> MNDQEKIDKFTHSYINDDFGLTIDQLVPKVKGYGRFNVWLGGNESKIRQVLKAVKEIGVSPTLFAVYEKNEGFSSGLGWLNHTSARGDYLTDAKFIARKLVSQSKQAGQPSWYDAGNIV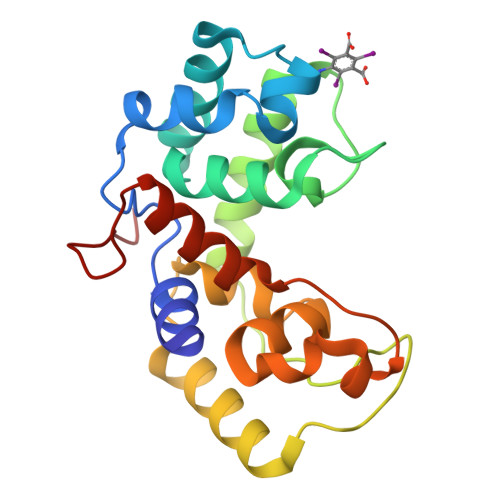HFVPQDVQRKGNADFAKNMKAGTIGRAYIPLTAAATWAAYYPLGLKASYNKVQNYGNPFLDGANTILAWGGKLDGKGGSPS> SRKIIHVDMDCFAAAVEMRDNPALRDIPIAIGGSRERRGVISCANYPARKFGVRSAMPTGMALKLCPHLTLLPGRFDAYKEASNHIREIFSRYTSRIEPLSLDEAYLDVTDSVHCHGSATLIAQEIRQTIFNELQLTASAGVAPVKFLAKIASDMNKPNGQFVITPAEVPAFLQTLPLAKIPGVGKVSAAKLEAMGLRTCGDVQKCDLVMLLKRFGKFGRILWERSQGIDERDVNSERLRKSVGVERTMAEDIHHWSECEAIIERLYPEL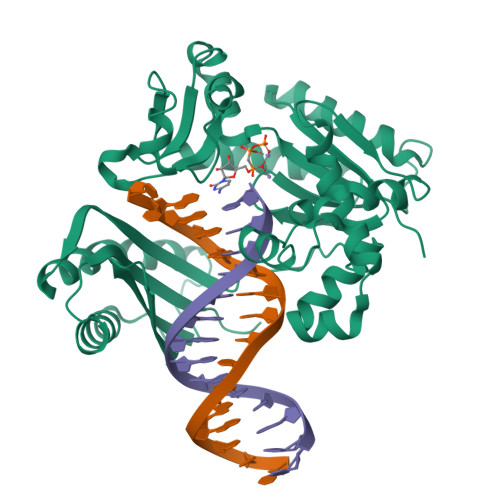ERRLAKVKPDLLIARQGVKLKFDDFQQTTQEHVWPRLNKADLIATARKTWDERRGGRGVRLVGLHVTLLDP;> GSRKIIHVDMDCFAAAVEMRDNPALRDIPIAIGGSRERRGVISCANYPARKFGVRSAMPTGMALKLCPHLTLLPGRFDAYKEASNHIREIFSRYTSRIEPLSLDEAYLDVTDSVHCHGSATLIAQEIRQTIFNELQLTASAGVAPVKFLAKIASDMNKPNGQFVITPAEVPAFLQTLPLAKIPGVGKVSAAKLEAMGLRTCGDVQKCDLVMLLKRFGKFGRILWERSQGIDERDVNSERLRKSVGVERTMAEDIHHWSECEAIIERLYPELERRLAKVKPDLLIARQGVKLKFDDFQQTTQEHVWPRLNKADLIATARKTWDERRGGRGVRLVGLHVTLLDP>AKGSTNHRALTGVIFEPFEEVKKELDLVPTVPQASLARQKYVDESESAVNEQINVEYNVSYVYHAMFAYFDRDNVALRGLAKFFKESSEEEREHAEKLMEYQNKRGGKVKLQSIVMPLSDFDHADKGDALHAMELALSLEKLTNEKLLNLHSV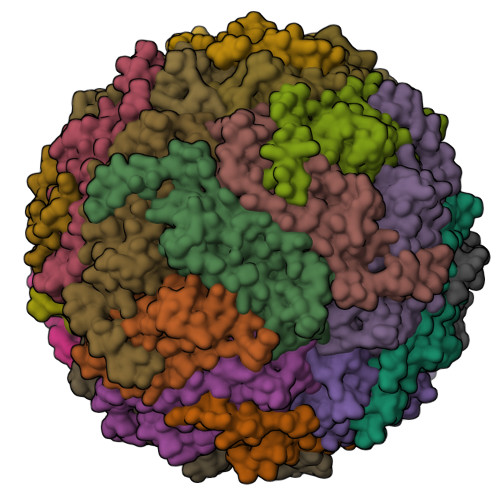ATKNGDVQLADFVETEYLGAQVEAIKRISEYVAQLRRVGKGHGVWHFDQMLLHEGGDAA[24x]>METFDQNEVDQILSEFHLQEEDLHVLMCRMQAEMERGLHLETNEEASVKMLPTYVRSTPDGSEVGDFLALDLGGTNFRVMLVKVGEDLEGQWKVETKHKMYSIPVDAMTGTAEMLFDYIAECISDYLDQQNMKHKKLPLGFTFSFPVRHEDIDKGILLNWTKGFKASGAEGNNVVGLLRDAIKRRGDFEMDVVAMVNDTVATMISCYYEDHHCEVGLIVGTGCNACYMEEMSNVELVEGEEGRMCVNTEWGAFGDTGELEDFRLEYDRVVDEASLNPGQQLYEKMIGGKYMGELVRLVLIKMVNENLLFGGESSEKLKTRGAFETQFVSQIEADTSDFKQTLNILRTLGVQATIGDCHAVRLACESVSTRAAIMCSAGLAGILNRMRQSRREELLRITVGVDGSVYKLHPSFKDKFHATVLKLTSGCEITFIQSEEGSGRGAALISAVAYKMAVMIGH[2x];>MRGTRKYQHVIETPDPGKWELAGYEESLPISEKSNPMTRELDKADPSQLVQLLRDCDAEIFQEEDENLIHYHRLYSESVLKTMGDVAKRVQEVLKNPDDSLVVLSGCGTSGRLALLLANSFNGLLKGLHKTPCYCYIMSGGDRSIVTSQESSED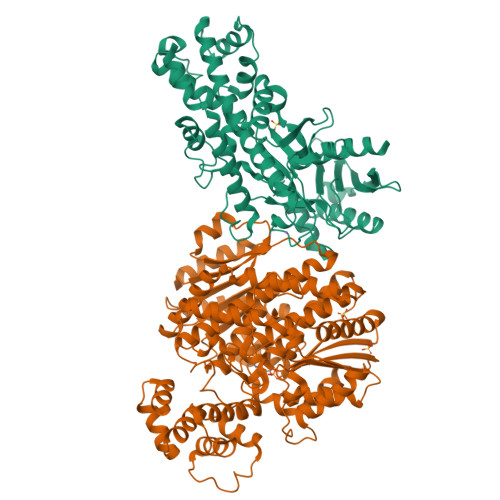NPQLGAQELEKVCEGKKNVLFIGISCGLSAPFIAGQLDFCMRHLDVYLPVLVGFNPVSMARNERIEGWHSSFRQVAERLQTLHDSQKGFILNPAVGPEGVSGSSRMKGGSATKILLETLLLVAHKAESNVPVTEKCLLEILRTYERAHKVTYSQSKKIAALMKQTATSLQKKGHLYILGWGTLGLVGIMDAVECVPTYQADWRDVRGFITGGYHSIENKEGDLSSLGPQFSISHEDFVKNVLPSVSETDTVLLIFTLDDDLNQIEKLVALVKEKTSNIQVICHATAGQYLPNSLKKTIPSIIGLTWPILFLEYEGAFIQKFQRELSTKWILDTVTSGAYTLRGKIFRNFMVDFKINNSKLFHRATSVLQRLTGQSQQRCTEVLLQSIYGEQTLSEQIRNTTIAGHVEAAASQDKVLPVAIVSLLRSCTIQDSRSRINSSLSIRSAIESSMNVPGRKRGAEDSESR[2x]> MSTGDSFETRFEKMDNLLRDPKSEVNSDCLLDGLDALVYDLDFPALRKNKNIDNFLSRYKDTINKIRDLRMKAEDYEVVK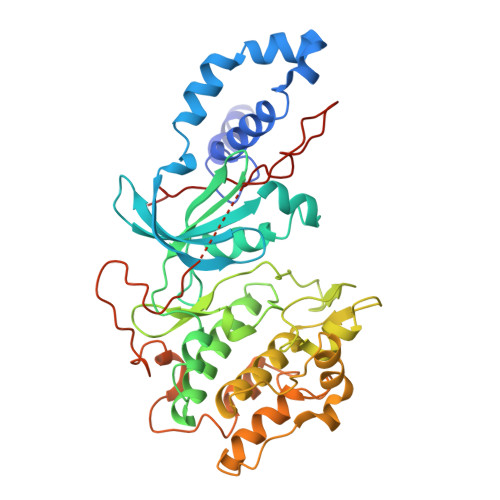VIGRGAFGEVQLVRHKSTRKVYAMKLLSKFEMIKRSDSAFFWEERDIMAFANSPWVVQLFYAFQDDRYLYMVMEYMPGGDLVNLMSNYDVPEKWARFYTAEVVLALDAIHSMGFIHRDVKPDNMLLDKSGHLKLADFGTCMKMNKEGMVRCDTAVGTPDYISPEVLKSQGGDGYYGRECDWWSVGVFLYEMLVGDTPFYADSLVGTYSKIMNHKNSLTFPDDNDISKEAKNLICAFLTDREVRLGRNGVEEIKRHLFFKNDQWAWETLRDTVAPVVPDLSSDIDTSNFDDLEEDKGEEETFPIPKAFVGNQLPFVGFTYYSNRRYL> GQDIQ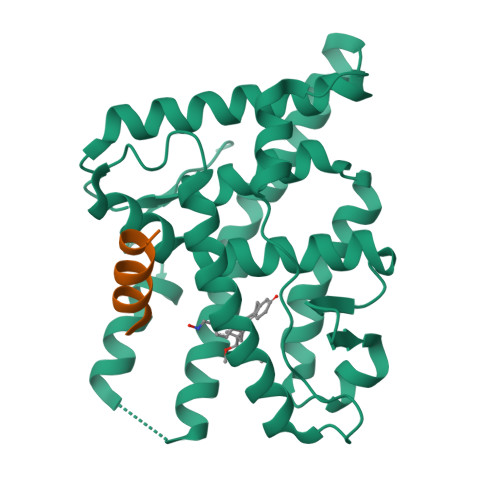LIPPLINLLMSIEPDVIYAGHDNTKPDTSSSLLTSLNQLGERQLLSVVKWSKSLPGFRNLHIDDQITLIQYSWMSLMVFGLGWRSYKHVSGQMLYFAPDLILNEQRMKESSFYSLCLTMWQIPQEFVKLQVSQEEFLCMKVLLLLNTIPLEGLRSQTQFEEMRSSYIRELIKAIGLRQKGVVSSSQRFYQLTKLLDNLHDLVKQLHLYCLNTFIQSRALSVEFPEMMSEVIAAQLPKILAGMVKPLLFHKK;> TNMGLEAIIRKALMGKY> ANIVGGIEYSINNASLCSVGFSVTRGATKGFVTAGHCGTVNATARIGGAVVGTFAARVFPGNDRAWVSLTSAQTLLPRVANGSSFVTVRGSTEAAVGAAVCRSGRTTGYQCGTITAKNVTANYAEGAVRGLTQGNACMGRGD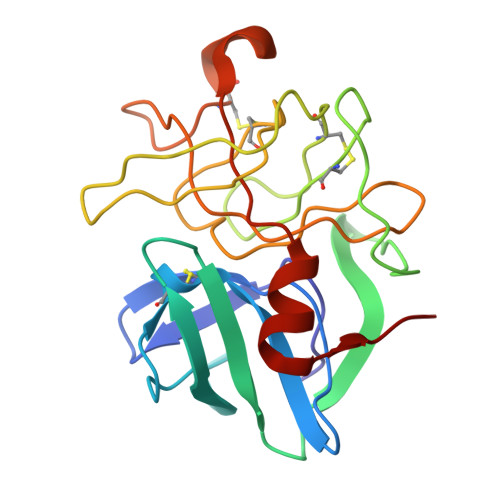SGGSWITSAGQAQGVASGGNVQSNGNNCGIPASQRSSLFERLQPILSQYGLSLVTG> MVEVKKHKFPGVYVVIDDDGSEKIATKNLVPGQRVYGERVIKWEGEEYRIWNPHRSKLGAAIVNGLKNFPIKPGKSVLYLGIASGTTASHVSDI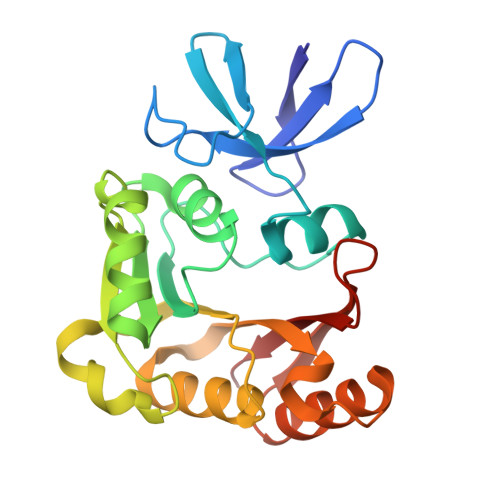VGWEGKIYGIEFSPRVLRELVPIVEERRNIIPILGDATKPEEYRALVTKVDVIFEDVAQPTQAKILIDNAKAYLKRGGYGMIAVKSRSIDVTKEPEQVFKEVERLLSEYFEVIERLNLEPYEKDHALFVVRKP> HQPST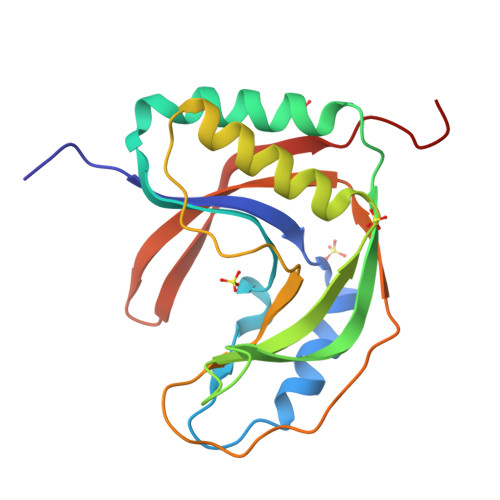YRLFYALRVPADITAPLAEAQAKLRGNWRAVRPDQMHVTLSYLPAVPPERVEDLKRLGTRLTQDLPPLHVNLRGTGYFPNEGSPRVWFVKTEAEGLTELAENLRAGIRELGIGTDDLAFKAHITLARKKGPAPRLPPLIFDQSWTAPGLTLYRSILRKTGPIYEVQSTFRFRGSASQ> SNAGKALVIVESPAKAKTINKYLGSDYVVKSSVGHIRDLPTS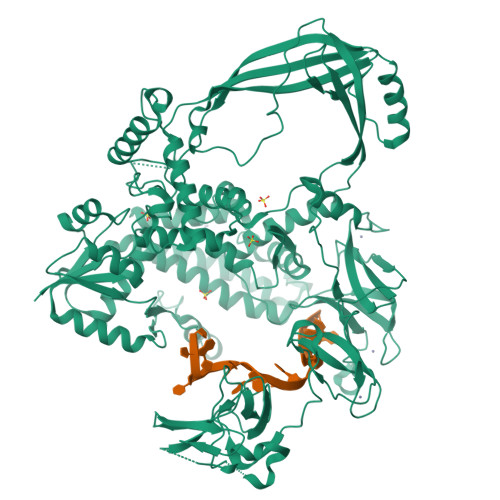GSAAKKSADSTSTKTAKKPKKDERGALVNRMGVDPWHNWEAHYEVLPGKEKVVSELKQLAEKADHIYLATDLDREGEAIAWHLREVIGGDDARYSRVVFNEITKNAIRQAFNKPGELNIDRVNAQQARRFMDRVVGYMVSPLLWKKIARGLSAGRVQSVAVRLVVEREREIKAFVPEEFWEVDASTTTPSGEALALQVTHQNDKPFRPVNKEQTQAAVSLLEKARYSVLEREDKPTTSKPGAPFITSTLQQAASTRLGFGVKKTMMMAQRLYEAGYITYMRTDSTNLSQDAVNMVRGYISDNFGKKYLPESPNQYASKENSQEAHEAIRPSDVNVMAESLKDMEADAQKLYQLIWRQFVACQMTPAKYDSTTLTVGAGDFRLKARGRILRFDGWTKVMPALRKGDEDRILPAVNKGDALTLVELTPAQHFTKPPARFSEASLVKELEKRGIGRPSTYASIISTIQDRGYVRVENRRFYAEKMGEIVTDRLEENFRELMNYDFTAQMENSLDQVANHEAEWKAVLDHFFSDFTQQLDKAEKDPEEGGMRPNQMVLTSIDCPTCGRKMGIRTASTGVFLGCSGYALPPKERCKTTINLVPENEVLNVLEGEDAETNALRAKRRCPKCGTAMDSYLIDPKRKLHVCGNNPTCDGYEIEEGEFRIKGYDGPIVECEKCGSEMHLKMGRFGKYMACTNEECKNTRKILRNGEVAPPKEDPVPLPELPCEKSDAYFVLRDGAAGVFLAANTFPKSRETRAPLVEELYRFRDRLPEKLRYLADAPQQDPEGNKTMVRFSRKTKQQYVSSEKDGKATGWSAFYVDGKWVEGKK>MAKKKKKKSFNVTRPTDPPVYPVTVPILGHIIQFGKSPLGFMQECKRQLKSGIFTINIVGKRVTIVGDPHEHSRFFLPRNEVLSPREVYSFMVPVFGEGVAYAAPYPRMREQLNFLAEELTIAKFQNFVPAIQHEVRKFMAANWDKDEGEINLLEDCSTMIINTACQCLFGEDLRKRLDARRFAQLLAKMESSLIPAAVFLPILLKLPLPQSARCHEARTELQKILSEIIIARKAAAVNKDSSTSDLLSGLLSAVYRDGTPMSLHEVCGMIVAAMFAGQHTSSITTTWSMLHLMHPANVKHLEALRKEIEEFPAQLNYNNVMDEMPFAERCARESIRRDPPLLMLMRKVMADVKVGSYVVPKGDIIACSPLLSHHDEEAFPEPRRWDPERDEKVEGAFIGFGAGVHKCIGQKFGLLQVKTILATAFRSYDFQLLRDEVPDPDYHTMVVGPTASQC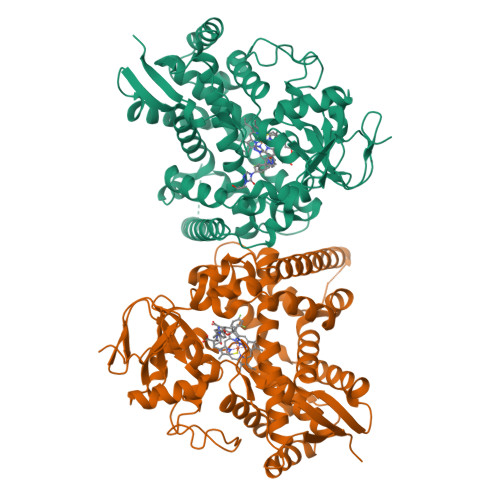RVKYIRRKAAAAHHHHHHHH[4x]> MKATWQSGQLTAELKRVTRLAAPMATVTIAQYLLPVISVMVAGHNGELQLSGVALATSFTNVTGFSIMYGLVGALETLCGQAYGAKQYEKIGTYTYSAIASNIPICFIISIIWFYIENILISLGQDPDISRIAGSYAFWLIPVLFAQAIVIPLTRFLLTQGLVLPLLYTAVTTLLFHVFVCWVFVLVFVLGSNGPAMATSVSFWFYAVILSCYVRFSSSCEKTRGFVSEDFVSCVKQFFQYGVPSAAMICLEWWLFELLILCSGLLSNPKLETSVLSICLTTETLHYVISSGVAAAVSTRVSNNLGAGNPQVARVSVLAGLCLWLVESAFFSILLFTFRNIIGYAFSNSKEVVDYVADLSPLLCLSFILDGFTAVLNGVARGSGWQHIGAWN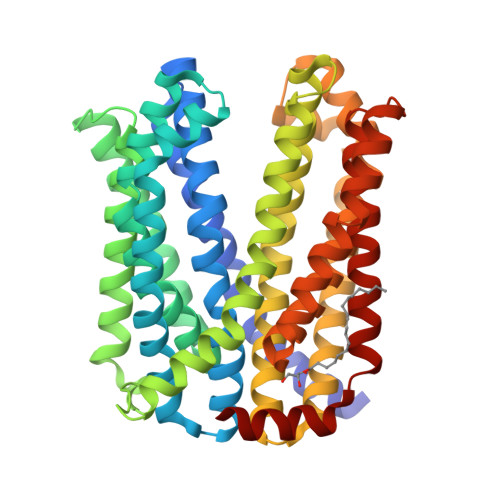NIFSYYLVGAPVGVYLAFRHDLNGKGLWCGVVIGSTVQATVLAIVTASMNWKEQAEKARKRIV>[2x]CGCAAATTI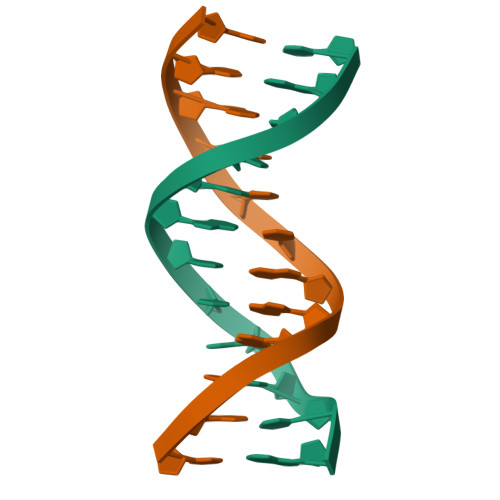GCG>[2x]MIIMEEAKKLIIELFSELAKIHGLNKSVGAVYAILYLSDKPLTISDIMEELKISKGNVSMSLKKLEELGFVRKVWIKGER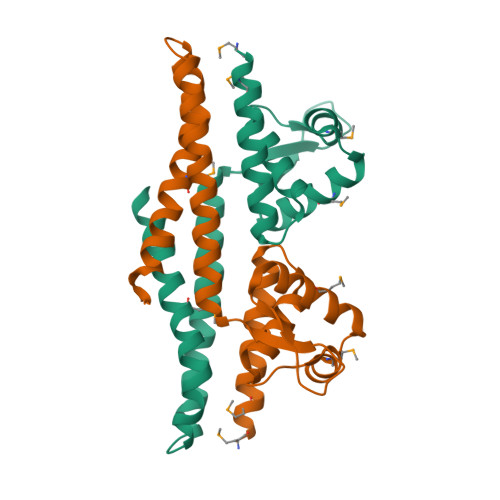KNYYEAVDGFSSIKDIAKRKHDLIAKTYEDLKKLEEKCNEEEKEFIKQKIKGIERMKKISEKILEALNDLDN>GPSTAGLGYGSWEIDPKDLTFLKELGTGQFGVVKYGKWRGQYDVAIKMIKEGSMSEDEFIEEAKVMMNLSHEKLVQLYGVCTKQRPIFIITEYMANGCLLNYLR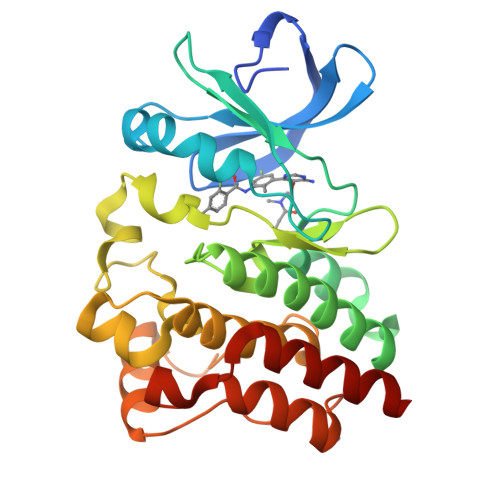EMRHRFQTQQLLEMCKDVCEAMEYLESKQFLHRDLAARNCLVNDQGVVKVSDFGLSRYVLDDEYTSSVGSKFPVRWSPPEVLMYSKFSSKSDIWAFGVLMWEIYSLGKMPYERFTNSETAEHIAQGLRLYRPHLASEKVYTIMYSCWHEKADERPTFKILLSNILDVMDEES[5x]>GSMGTP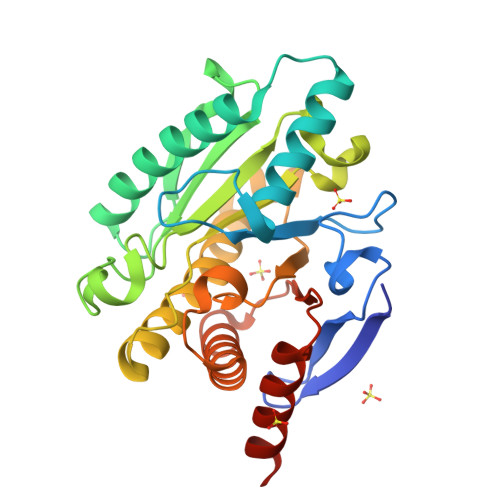DPLTLRFTCLGDRNVIFFGPSGRQDGFTPLYDPSPSKRVATVDAGTYGLFIGGVGMNGEFADTIIEEARRNRIPLTATELSAESQEIQERLLHDAERQPGTLVEIDSGRFSRVFARSFAYVAIVPNTVWDESETGKNVGATFLHILKPEVTPHGNEMNDVMLYTVAPFGNASDSAYNMAYKATMLGIVGAVSEYNKTPWGEVKPVEAIRLPLLGAGHFRGRRGLHSIGRANAVAVEAAITRFDPRVELQFMYEPSDTALRGLMESERKYKFPQGD[3x]Trypanothione reductase (TR) is a key factor in the redox homeostasis of trypanosomatid parasites, critical for survival in the hostile oxidative environment generated by the host to fight infection. In the case of the Trypanosomatidae, redox homeostasis relies on the dithiol trypanothione (TSH), a peculiar variant of glutathione (GSH) in which two GSH molecules are joined by the polyamine spermidine. TSH is kept in the reduced state by the action of the NADPH/FAD-dependent protein trypanothione reductase, homolog to the human glutathione reductase (GR). TR is considered an attractive target for the development of new trypanocidal agents as it is essential for parasite survival but has no close homolog in humans.

Crystallographic fragment screening performed at the XChem facility allowed us to test 352 small compounds from the DSiP library, a collection specifically designed to ensure rapid and cheap follow-up synthesis. Data analysis, performed by the PanDDA algorithm, reported 480 interesting “events” clustered in 33 sites possibly associated to fragment binding. Visual inspection of these putative events led to the identification of 21 true binding events in eight sites, corresponding to 12 fragment hits distributed in 5 independent binding sites, described later in detail. All datasets have a resolution higher than 2 Å and the modeled fragments show a good correlation with the electron density maps, as proven by the real-space correlation coefficient (RSCC). Indeed, the RSCC is around 0.9 for most hits and always in the range of 0.77–0.93.

>[2x]GSHMSKAFDLVVIGAGSGGLEAGWNAATLYGKRVAVVDVQTSHGPPFYAALGGTCVNVGCVPKKLMVTGAQYMDHLRESAGFGWEFDGSSVKANWKKLIAAKNEAVLDINKSYEGMFNDTEGLDFFLGWGSLESKNVVVVRETADPKSAVKERLQADHILLATGSWPQMPAIPGIEHCISSNEAFYLPEPPRRVLTVGGGFISVEFAGIFNAYKPPGGKVTLCYRNNLILRGFDETIREEVTKQLTANGIEIMTNENPAKVSLNTDGSKHVTFESGKTLDVDVVMMAIGRIPRTNDLQLGNVGVKLTPKGGVQVDEFSRTNVPNIYAIGDITDRLMLTPVAINEGAALVDTVFGNKPRKTDHTRVASAVFSIPPIGTCGLIEEVAAKEFEKVAVYMSSFTPLMHNISGSKYKKFVAKIVTNHSDGTVLGVHLLGDGAPEIIQAVGVCLRLNAKISDFYNTIGVHPTSAEELCSMRTPSYYYVKGEKMEKLPDSNL>SEQETRGANEAIDFNDELRNRREKLAALRQQGVAFPNDFRRDHTSDQLHEEFDAKDNQELESLNIEVSVAGRMMTRRIMGKASFVTLQDVGGRIQLYVARDSLPEGVYNDQFKKWDLGDIIGARGTLFKTQTGELSIHCTELRLLTKALRPLPDKFHGLQDQEVRYRQRYLDLIANDKSRQTFVVRSKILAAIRQFMVARGFMEVETPMMQVIPGGASARPFITHHNALDLDMYLRIAPELYLKRLVVGGFERVFEINRNFRNEGISVRHNPEFTMMELYMAYADYHDLIELTESLFRTLAQEVLGTTKVTYGEHVFDFGKPFEKLTMREAIKKYRPETDMADLDNFDAAKALAESIGITVEKSWGLGRIVTEIFDEVAEAHLIQPTFITEYPAEVSPLARRNDVNPEITDRFEFFIGGREIGNGFSELNDAEDQAERFQ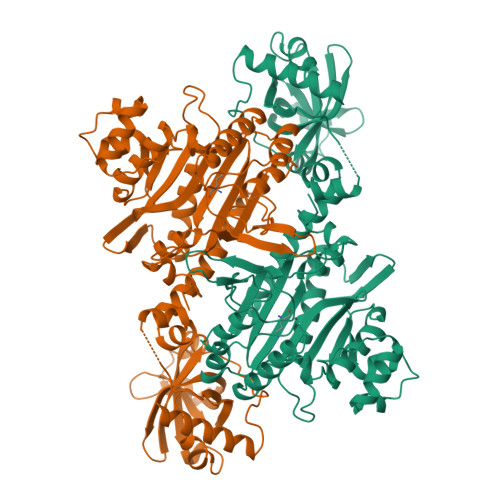EQVNAKAAGDDEAMFYDEDYVTALEYGLPPTAGLGIGIDRMIMLFTNSHTIRDVILFPAMRPQK[3x]> MIFAVRTMVGQEKNIAGLMASRAEKEQLDVYSILASESLKGYVLVEAETKGDVEELIKGMPRVRGIVPGT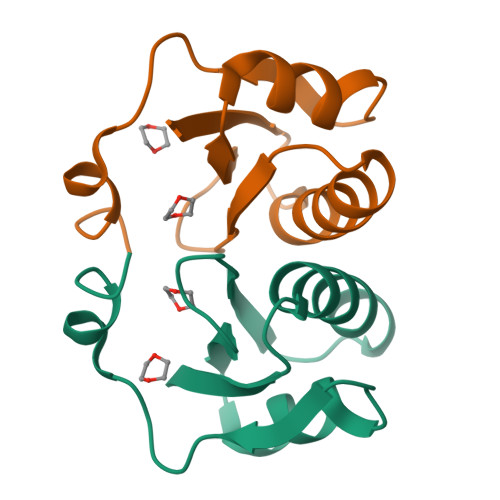IAIEEIEPLLTPKLEHHHHHH>[2x]MPYHEFEVSKCIPERREHAVMKAAGEDLTSCLPKGYLNTIPGTISERGCAYCGAKHVIGTPMKDVIHISHGPNGCTYDTWQTKRYISDNDNFQLKYTFATDVKE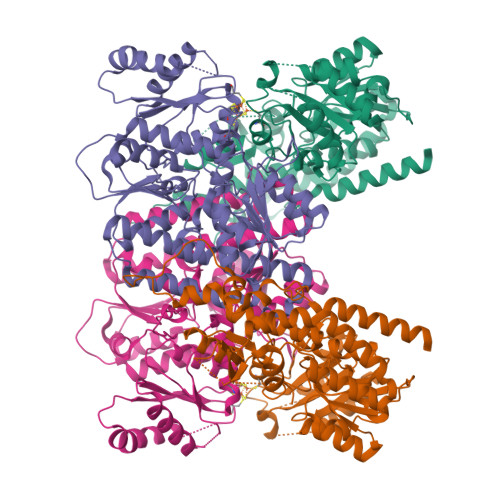KHVVFGAEGLLKKSMHEAFDAFPNIKRMTVYQTCTTALIGDDVDAIAKEVMEERGDVDVFVCNSPGFAGPSQSGGHHKINIAWLNQKVGTVEPDYLGEHVINYVGEYNIQGDQEVMIDYFNRMGIQVLSTFTGNGSYDSLRMMHRAHLNVLECARSAEYICDELRARYGIPRLDIDGFGFEPLANSLRKVALFFGIEDKAEAIIAEEYAKWKPQLDWYKERLKGKKVCLWPGGSKLWHWAHAIEEEMGLKVVSVYTKFGHQGDMEKGVSRCGEGALAIDDPNELESVEAIEMLKPDIIFTGKRPGEFVKKHGVPYLNAHAYHNGPYKGFEGWVRFARDIYNAIYSPMRQLAALDISAPDAAITSGFRTAKMNADLTVSDEVKFSEVLHEYTGKYDSIAEIRARNQAYAAEQKALRDAVQPAAEWSHPQFEK;>MTCQVTQKAREGTINPIFTCQPAGAQFASIGIKDCIGIVHGGQGCVMFVRLLISQHMKESFEIASSSVHEDGAVFGALDRVETAVEVLLTRYPDVKVVPIITTCSTEIIGDDVDGLLSKLEDELLPTKFPGREVHLLTVHCPSFVGSMITGYDKAVHDFVKKFATKDEPSDKINLITGWVNPGDVKELKHLLEVMEVKANVLFEVESFDSPLMPDLEHHSHGSTTIEDLRDTANAKGTIALNRYEGMKAADYLKKKFKVPAVIGPTPVGIRNTDAFLKAVSEMTGQPIPAQLVKERGLALDAIADIGHMFLADKRVAIYANPDLAIGLTEFCLDLEMKPKLLLLGDDNSGYVKDPRVLALQENAPDLEIVTNADFWDLESRIQQGLELDLILGHSKGRFISIDYKVPMVRVGFPTYDRAGMYRHPVLGYGGAMFLAETMANTLFADMEAKKNKEWILNVW[2x]> MYQLQFINLVYD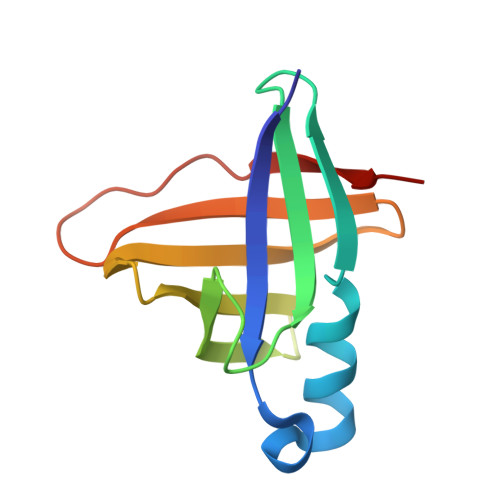TTKLTHLEQTNINLFIGNWSNHQLQKSICIRHGDDTSHNQYHILFIDTAHQRIKFSSFDNEEIIYILDYDDTQHILMQTSSKQGIGTSRPIVYERLV>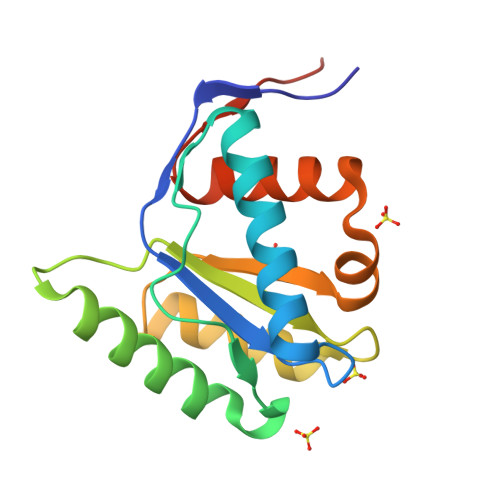 MNKKMINGGTVNNWICINFSRQVQDNLARTFCQELAQMCYVSGMAFNPEPVLPPVSARPEQVEKVLKTRYHDATSKLSQGKEIDLLIVILPDKKNSDLYGDLKRICETELGIVSQCCLTKHVFKMSKQYMANVALKINVKVGGRNTVLVHHHHHH> MPLDTSTYKLALLRVDGRRWNELRRVHAQIRTQAAADGSSYLEMGHTKVMCVVTGPSEPGPRRGTGAGTTGGGGAGGAGGGGSGGQGKEAEVVVSIVIAGFSSVDRKRHGRND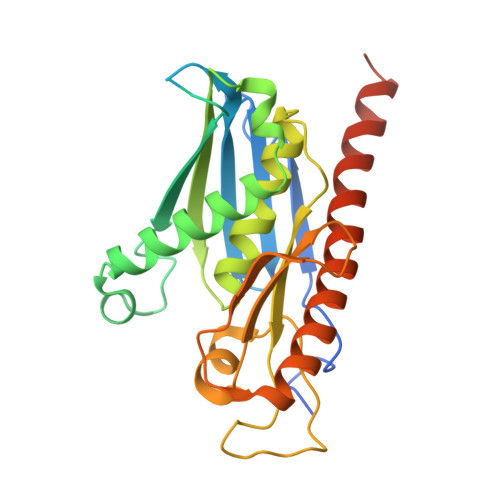KRIIEMQSTVANALSASLHTHLFPHSQITISLHVLSQDGSLLAALINAATLACVDAGIPMTDYVVACTAGSTSTYAANDENADPLLDLNHQEEQELPWLTVATLGESDKVAVLVCESRVQVSRLEGMLAVGVDGCKQIRAILDHVVRQKGRRMIREGAVEKGVSLDDMDED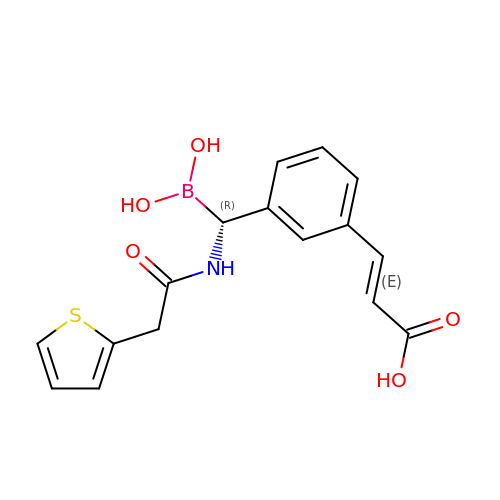(1R)-1-(2-THIOPHEN-2-YL-ACETYLAMINO)-1-(3-(2-CARBOXYVINYL)-PHENYL) METHYLBORONIC ACID | C16 H16 B N O5 S | ZDYRJUZJSKGVDJ-MOEXGYKKSA-N>[3x]PPGPPGPPGLPGQ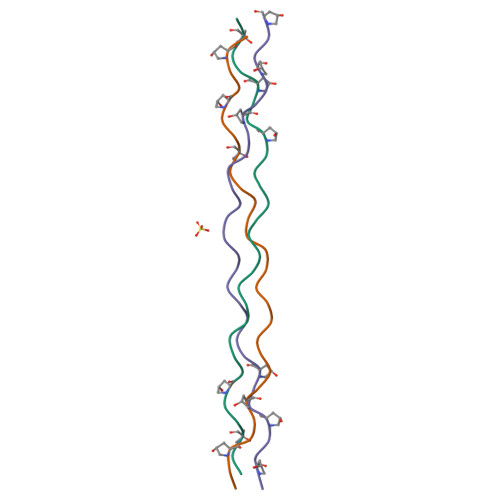RGERGFPGPPGPPGPPG>AEPQPPSGGLTDEAALSCCSDADPSTKDFLLQQTMLRVKDPKKSLDFYTRVLGMTLIQKCDFPIMKFSLYFLAYEDKNDIPKEKDEKIAWALSRKATLELTHNWGTEDDETQSYHNGNSDPRGFGHIGIAVPDVYSACKRFEELGVKFVKKPDDGKMKGLAFIQDPDGYWIEILNPNKMATLM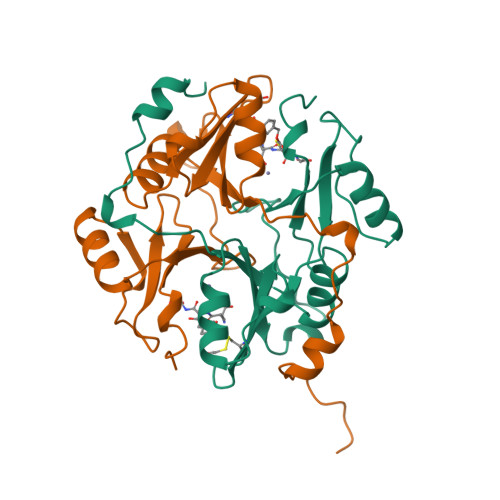[4x]> VP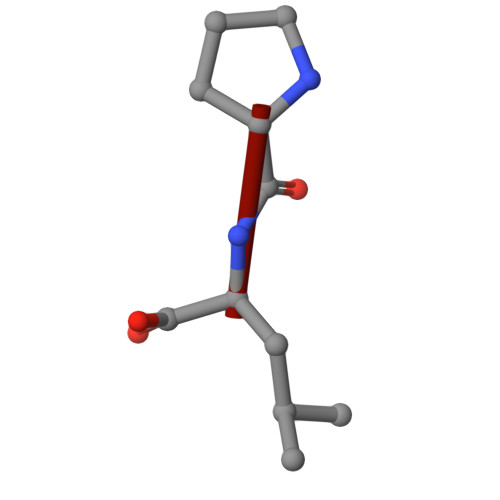L> GIDPFTGQKLDFFKQAHEGGPAPNSEVVRPDGFQSQRILDYAQGTRPLVLNFGSCTCP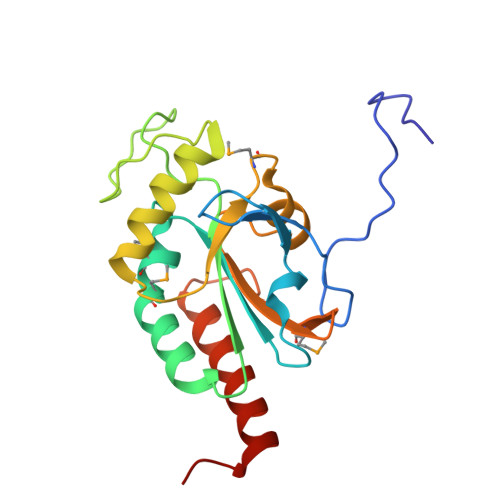PFMARMSAFQRLVTKYQRDVDFLIIYIEEAHPSDGWVTTDSPYVIPQHRSLEDRVSAARVLQQGAPGCALVLDTMANSSSSAYGAYFERLYVIQSGTIMYQGGRGPDGYQVSELRTWLERYDEQLHGTRPHRF> GPLGSMTTDEGAKNNEESPTATVAEQGEDITSKKDRGVLKIVKRVGNGEETPMIGDKVYVHYKGKLSNGKKFDSSHDRNEPFVFSLGKGQVIKAWDIGVATMKKGEICHLLCKPEYAYGSAGSLPKIPSNATLFFEIELLDFKGEDLFEDGGIIRRTKRKGEGYSNPNEGATVEIHLEGRCGGRMFDCRDVAFTVGEGEDHDIPIGIDKALEKMQREEQCILYLGPRYGFGEAGKPKFGIEPNAELIYEVTLKSFEKAKESWEMDTKEKLEQAAIVKEKGTVYFKGGKYMQAVIQYGKIVSWLEMEYGLSEKESKASESFLLAAFLNLAMCYLKLREYTKAVECCDKALGLDSANEKGLYRRGEAQLLMNEFESAKGDFEKVLEVNPQNKAARLQISMCQKKAKEHNERDRRIYANMFKKFAEQDAKEEANKAMGKKTSEGVTNEKGTDSQAMEEEKPEGHV;> HHHHHHDDTSRMEEVD

FKBP51 is the co-chaperone to Hsp90 and belongs to the immunophilin family initially recognized for its involvement in regulation of steroid hormone receptor activity. Going from the N-terminus to C-terminus, the overall FKBP51 structure contains two mixed beta sheet wrapped around a central helix for FK1 and FK2 domains followed by the TPR domain consisting of three TPR repeats and one additional long helix in the C-terminus. FK1 domain is active as PPIase and known to bind to the FK506 and rapamycin inhibitors or modulators. Inside the cell, the TPR domain of FKBP51 mediates interaction with EEVD C-terminal sequence of Hsp90/Hsp70 molecular chaperones.

Interestingly, we observed that out of 9 amino acids, all except one are involved in some kind of interactions with the TPR binding pocket. The valine and methionine side chains of the C90 peptide are buried into hydrophobic pockets contributing to the complex formation. It is also observed that the C-terminal aspartate (Asp732) is involved in formation of the di-carboxylate clamp with the help of hydrogen bonding and salt bridges. The results indicated that the Asp732 nitrogen formed a hydrogen bond with the OD1 atom of carboxylate group of Asn322 with a distance of 2.78 Å. Asp732 is also interacting to Lys272 and Lys352 with the help of three salt bridges SB1, SB2 and SB3 with a length of 3, 3.39 and 3.70 Å, respectively. The fourth salt bridge SB4, is formed between Glu729 and Lys329 at a distance of 2.79 Å. Glu730 was involved in formation of hydrogen bonds, HB3, HB4, HB5, and HB6 with Lys352 and Arg356 with a length of 2.91, 2.78, 3.33 and 3.29 Å, respectively. We run the Vasco software that enables to display the electrostatic and hydrophobic surface and observed that in the complex surface the concave groove in the TPR domain is positively charged which makes long range attractions for the negatively charged C90 peptide. Similarly, for the complex structure we obtained a resolution of 2.49 Å with 62% spherical completeness.Nuclear receptor coactivator 7 (NCOA7) belongs to the TLDc [Tre2/Bub2/Cdc16 (TBC), lysin motif (LysM), domain catalytic] domain-containing family of proteins. The human NCOA7 gene encodes several mRNA isoforms; among these, isoform 4, named NCOA7-AS, is up-regulated by type 1 interferon in response to viral infection. NCOA7 and NCOA7-AS both interact with several subunits of the vacuolar proton pump V-ATPase, which leads to increased acidification of the endolysosomal system and consequently impairs infection by viruses that enter their host cells through the endosomal pathway, such as influenza A virus and hepatitis C virus. Similarly to full-length NCOA7, NCOA7-AS possesses a TLDc domain in its C-terminus.

Here, we report the crystal structure of the TLDc domain of the human NCOA7-AS protein at high resolution. NCOA7-AS has a tendency to aggregate and to form large oligomers as judged by size-exclusion chromatography (SEC). We therefore alternatively expressed and purified a truncated form of NCOA7-AS corresponding to the TLDc domain, hereafter referred to as TLDcHs, using E. coli as an expression host. A full X-ray data set could be collected and processed to a resolution of 1.8 Å. Most residues could be rebuilt for the six monomers, except for the first two amino acids of chain A and the first three residues at the N-terminus for chains B, C, D, F and E. Gly175 was not modeled in chain A as well as the glycine stretch ranging from 174 to 176 in chain F. Residues 146–148 were also disordered in chain F but were well ordered in the other chains. Analysis of the crystal packing with the PISA server revealed the potential existence of a stable complex made of three TLDcHs monomers within the asymmetric unit. The overall structure of TLDcHs is globular and consists of two α-helices in the N-terminus and ten β-strands forming two antiparallel β-sheets. The two sheets, organized as a central pseudo-orthogonal β-sandwich, are made by strands β1, β2, β3, β4, β5 and β10 and strands β6, β7, β8 and β9, respectively. The fold is similar to those of the two previously solved TLDc structures from D. rerio OXR2 (TLDcDr) and D. melanogaster TBC1D24 (TLDcDm). TLDcHs shares 62% sequence identity with TLDcDr and the two structures display an r.m.s.d. of 0.7 Å when superposed over 164 Cα atoms.

>GMRPHSALLENMHIEQLARRLPARVQGYPWRLAYSTLEHGTSLKTLYRKSASLDSPVLLVIKDMDNQIFGAYATHPFKFSDHYYGTGETFLYTFSPHFKVFKWSGENSYFINGDISSLELGGGGGRFGLWLDADLYHGRSNSCSTFNNDILSKKEDFIVQDLEVWAFD[6x]>APSRKFFVGGNWKMNGRKKNLGELITTLNAAKVPADTEVVCAPPTAYIDFARQKLDPKIAVAAQNCYKVTNGAFTGEISPGMIKDCGATWVVLGHSERRHVFGESDELIGQKVAHALSEGLGVIACIGEKLDEREAGITEKVVFEQTKVIADNVKDWSKVVLAYEPVWAIGTGKTATPQQAQEVHEKLRGWLKSNVSDAVAQSTRIIYGGSVTGATCKELASQPDVDGFLVGGASLKPEFVDII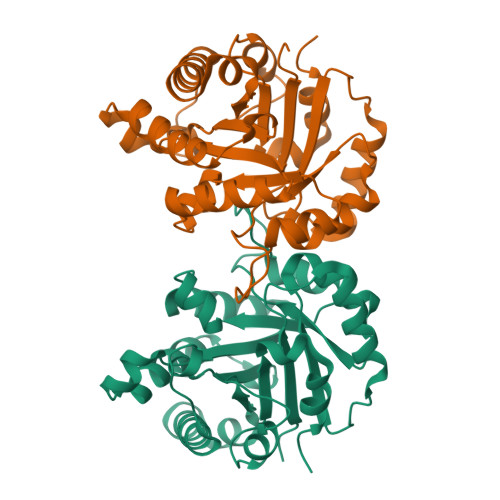NAKQ[2x]> MNAGSDPVVIVSAARTIIGSFNGALAAVPVQDLGSTVIKEVLKRATVAPEDVSEVIFGHVLAAGCGQNPVRQASVGAGIPYSVPAWSCQMICGSGLKAVCLAVQSIGIGDSSIVVAGGMENMSKAPHL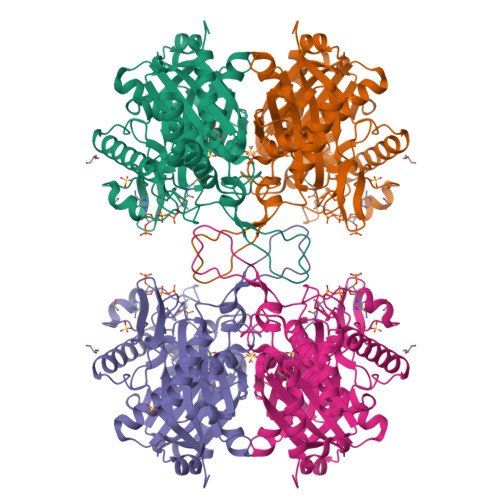AYLRTGVKIGEMPLTDSILCDGLTDAFHNCHMGITAENVAKKWQVSREDQDKVAVLSQNRTENAQKAGHFDKEIVPVLVSTRKGLIEVKTDEFPRHGSNIEAMSKLKPYFLTDGTGTVTPANASGINDGAAAVVLMKKSEADKRGLTPLARIVSWSQVGVEPSIMGIGPIPAIKQAVTKAGWSLEDVDIFEINEAFAAVSAAIVKELGLNPEKVNIEGGAIALGHPLGASGCRILVTLLHTLERMGRSRGVAALCIGGGMGIAMCVQRE> MPNPSPPSSSSPVQTLISILRIIPDWSDRTQERGMRQHRTLYDHEKWMHHRSSYRHLRHLLSSLSSRVILSLIPPVIAFTLVAVVIASYNTAVALDLLPGIFPLLRSSSLPYQLTAPALALLLVFRTEASYSRFEEGRKSWTEVIAGANDFARQIISSVETSGDAQLKKALLQYIVAFPVALKCHVIYGSDIARDLQNLLEVDDLLVVLNSKHRPGCIIQFISRSLQLLKLEESRRIMLQSKISCFHEGIGICEQLIGTPIPLSYTRLTSRFLVLWH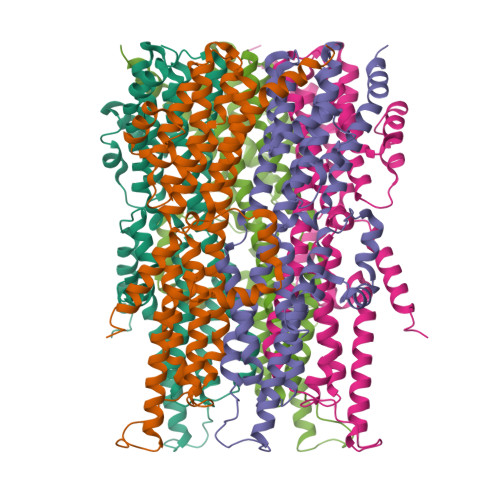LTLPIILWDDCHWIVVPATFISAASLFCIEQVGVLIEEPFPMLALDDLCNSVRNNVQEALASEKLIRARLAAKGRIQSEQQFQNGQPRPENLYFQ> HHHHHHMGKYNLILSEYLSFIYNSQSAVQIPIYYSSNSELENRCIEFHSKCLENSKNGLSLRKLFVEYNDVIENATLLSILSYSYDKYNAVERKLVKYAKGKPLEADLTVNELDYENNKMTSELFPTAEEYTDSLMDPAILTSLSSNLNAVMFWLEKHENDVAEKLKVYKRRLDLFTIVASTINKYGVPRHNAKYRYEYDVMKDKPYYLVTWANSSIEMLMSVFSHDDYLIAKELIVLSYSNRSTLAKLVSSPMSILVALVDINGTFITNEELELEFSNKYVRAIVPDQTFDELNQMLDNMRKAGLVDIPKMIQDWLVDRSIEKFPLMAKIYSWSFHVGFRKQKMLDAALDQLKTEYTENVDDEMYREYTMLIRDEVVKMLEEPVKHDDHLLRDSELAGLLSMSSASNGESRQLKFGRKTIFSTKKNMHVMDDMANERYTPGIIPPVNVDKPIPLGRRDVPGRRTRIIFILPYEYFIAQHAVVEKMLIYAKHTREYAEFYSQSNQLLSYGDVTRFLSNNTMVLYTDVSQWDSSQHNTQPFRKGIIMGLDILANMTNDAKVLQTLNLYKQTQINLMDSYVQIPDGNVIKKIQYGAVASGEKQTKAANSIANLALIKTVLSRISNKHSFATKIIRVDGDDNYAVLQFNTEVTKQMIQDVSNDVRETYARMNAKVKALVSTVGIEIAKRYIAGGKIFFRAGINLLNNEKRGQSTQWDQAAILYSNYIVNRLRGFETDREFILTKIMQMTSVAITGSLRLFPSERVLTTNSTFKVFDSEDFIIEYGTTVDEVYIQRAFMSL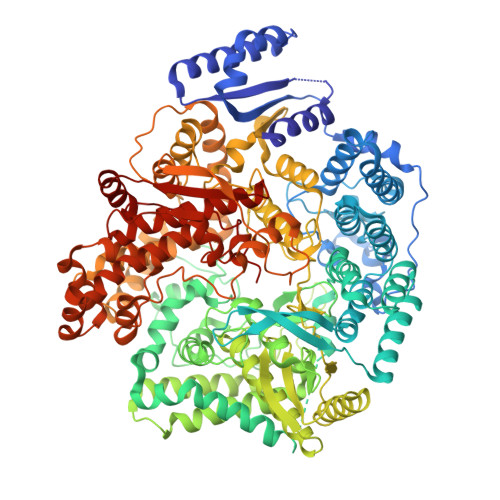SSQKSGIADEIAASSTFKNYVTRLSEQLLFSKNNIVSRGIALTEKAKLNSYAPISLEKRRAQISALLTMLQKPVTFKSSKITINDILRDIKPFFTVSDAHLPIQYQKFMPTLPDNVQYIIQCIGSRTYQIEDDGSKSAISRLISKYSVYKPSIEELYKVISLHENEIQLYLISLGIPKIDADTYVGSKIYSRDKYRILESYVYNLLSINYGCYQLFDFNSPDLEKLIRIPFKGKIPAVTFILHLYAKLEVINYAIKNGSWISLFCNYPKSEMIKLWKKMWNITSLRSPYTNANFFQEP>MKPQKIVIKLGMPSPKNRTKAMVLAAKVYGVSSVAITGDDKDQLEVVGVDVDTACLVSCLRKK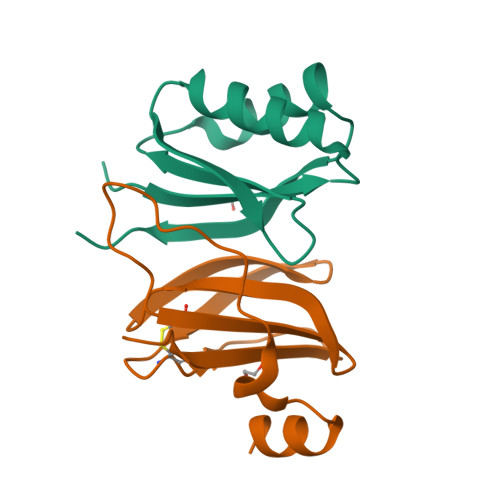VLRRADIMVVEEAKDK[8x];>GPMQNEYIDAKKHGIDLSRERAPNFVDHPGIPPSDCFWFLYKNYVRQNAGVCQSDWSFDMKIGQYWVTIHTDEGCRLSGIIPAGWLILGMKRPGF[8x]>MVEEVSNKQ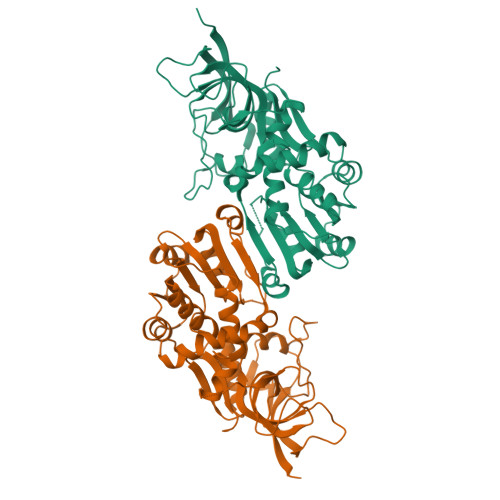IIFKDYINGFPKESDMILKTSTIKLKVPEGCNDAVLVKNLYLSCDPYMRSRMSKLDDNYVPIFIPGSPITGDGVAKVLDSSHPDFKRGDLIRGITGWEEYTLIQSAEFITKIQHTDLPLSYHIGILGMPGLTAYAGFYEISSPKEGETVFVSAASGAVGQLVGQFAKLSGCYVVGSAGTKDKVDMLKNKFGFDDAFNYKEEHDLDAALKRYFPEGIDIYFDNVGGKMLDAVLPNMKTKGRIATCGMISQYNLDEAEGVRNLFCIMTKQIRMQGYLVYYYRHLYPKLFDLVVPLLRQGKINYVEDVAEGLESAPAALIGLFSGRNVGKQVVRVATE[2x]> MTTQSPLNSFYATGTAQAVSEPIDVESHLGSITPAAGAQGSDDIGYAIVWIKDQVNDVKLKVTLANAEQLKPYFKYLQIQITSGYETNST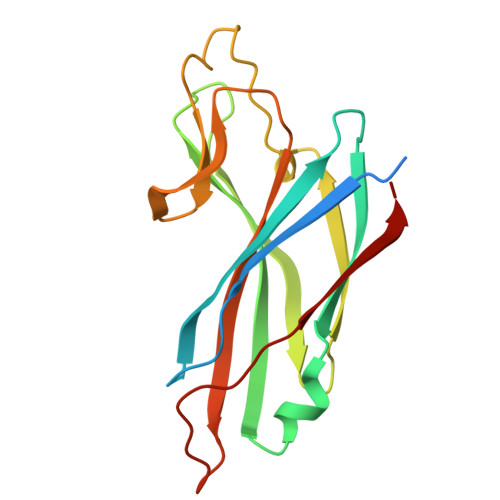ALGNFSETKAVISLDNPSAVIVLDKEDIAVLYPDKTGYTNTSIWVPGEPDKIIVYNETKPVAILNFKAFYEAKEGMLFDSLPVIFNFQVLQVG> GSGGIEGAISVGSSIVGQSPYKFGGGRTQSDINNRI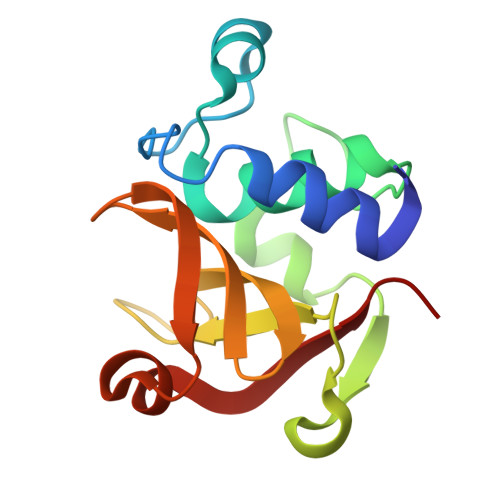FDCSSFVRWAYASAGVNLGPVGGTTTDTLVGRGQAVSASEMKRGDLVFFDTYKTNGHVGIYLGNGTFLNDNTSHGVSVDSMSNPYWKAAFKGVVRRVVQ>MSKPQPIAAANWKCNGSQQSLSELIDLFNSTSINHDVQCVVASTFVHLAMTKERLSHPKFVIAAQNAIAKSGAFTGEVSLPILKDFGVNWIVLGHSERRAYYGETNEIVADKVAAAVASGFMVIACIGETLQERESGRTAVVVLTQIAAIAKKLKKADWAKVVIAYEPVWAIGTGKVATPQQAQEAHALIRSWVSSKIGADVRGELRILYGGSVNGKNARTLYQQRDVNGFLVGGASLKPEFVDIIKATQ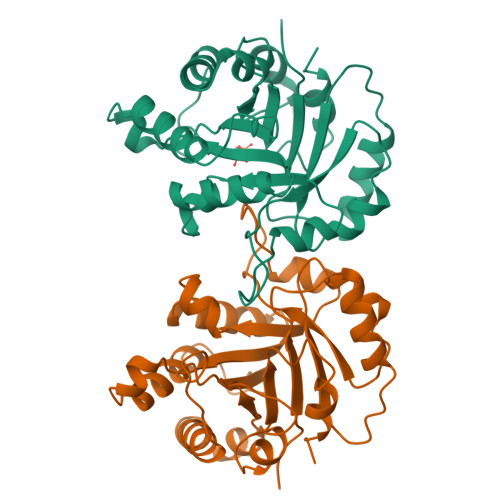[2x]> MGFETVVPAPPTRDDELRMIKATEEQFLQQPRYKLYMNEAHRIAKMNHGDRHNNIRAHFWSNFALGLLITGPIFIIPFGKAFRNLRSGVPYYFRPKYVFTQKN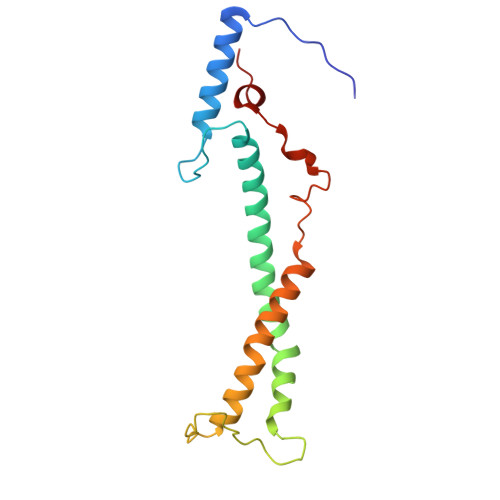QYNQDRNWGAMKKQIPLWLGLSTAYAYWFTDFSINDDEWLEKGKVIYPHQTIKVL> MDPV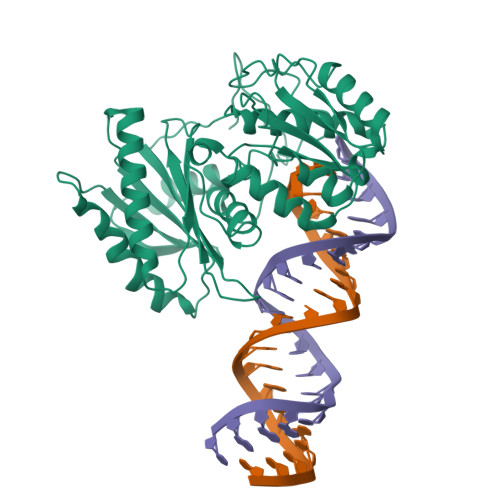RPLFRGPTPVHPSQCVRMPGCWPQAPRPLEPAWGRAGPAGRGLVFRKPEDSSPPLQPVQKDSVGLVSMFRGMGLDTAFRPPSKREVPPLGRGVLGRGLSANMVRKDREEPRSSLPDPSVLAAGDSKLAEASVGWSRMLGRGSSEVSLLPLGRAASSIGRGMDKPPSAFGLTARDPPRLPQPPALSPTSLHSADPPPVLTMERKEKELLVKQGSKGTPQSLGLNLIKIQCHNEAVYQYHVTFSPSVECKSMRFGMLKDHQSVTGNVTAFDGSILYLPVKLQQVVELKSQRKTDDAEISIKIQLTKILEPCSDLCIPFYNVVFRRVMKLLDMKLVGRNFYDPTSAMVLQQHRLQIWPGYAASIRRTDGGLFLLADVSHKVIRNDSVLDVMHAIYQQNKEHFQDECSKLLVGSIVITRYNNRTYRIDDVDWNKTPKDSFVMSDGKEITFLEYYSKNYGITVKEDDQPLLIHRPSERQNNHGMLLKGEILLLPELSFMTGIPEKMKKDFRAMKDLTQQINLSPKQHHGALECLLQRISQNETASNELTRWGLSLHKDVHKIEGRLLPMERINLRNTSFVTSEDLNWVKEVTRDASILTIPMHFWALFYPKRAMDQARELVNMLEKIAGPIGMRISPPAWVELKDDRIETYIRTIQSLLGVEGKIQMVVCIIMGTRDDLYGAIKKLCCVQSPVPSQVINVRTIGQPTRLRSVAQKILLQMNCKLGGELWGVDIPLKQLMVIGMDVYHDPSRGMRSVVGFVASINLTLTKWYSRVVFQMPHQEIVDSLKLCLVGSLKKYYEVNHCLPEKIVVYRDGVSDGQLKTVANYEIPQLQKCFEAFDNYHPKMVVFVVQKKISTNLYLAAPDHFVTPSPGTVVDHTITSCEWVDFYLLAHHVRQGCGIPTHYICVLNTANLSPDHMQRLTFKLCHMYWNWPGTIRVPAPCKYAHKLAFLSGQILHHEPAIQLCGNLFFL> SMGAEPGRPARLDQLLDMPAAGLAVQLRHAWNPEDRSLNVFVKDDDRLTFHRHPVAQSTDGIRGKVGHARGLHAWQINWPARQRGTHAVVGVATARAPLHSVGYTALVGSDAESWGWDLGRSRLYHDGKNQPGVAYPAFLGPDEAFALPDSLLVVLDMDEGTLSFIVDGQYLGVAFRGLKGKKLYPVV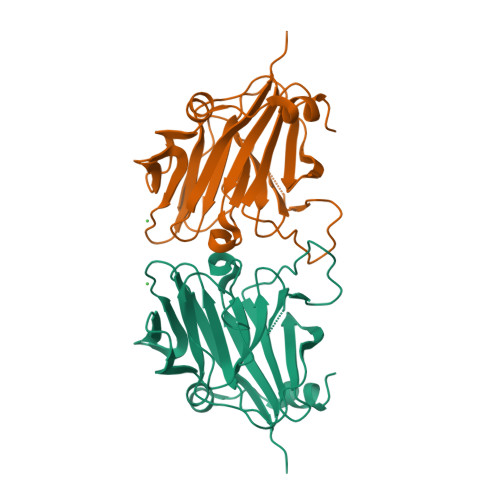SAVWGHCEVTMRYINGLDPE> GSHMRFDEFGNIITDSAVAEEPEPELPGVTEEALRLKEAALEELAAQEVTAPLVPLAVSAFLTSRKKAAAAELADWMQSPEGQASSLESIGRSLSRRNHGRSRAVVLAHDHDEAIKGLRAVAAGKQAPNVFSVDGPVTTGPVWVLAGFGAQHRKMGKSLYLRNEVFAAWIEKVDALVQDELGYSVLELILDDAQDYGIETTQVTIFAIQIALGELLRHHGAKPAAVIGQSLGEAASAYFAGGLSLRDATRAICSRSHLMGEGEAMLFGEYIRLMALVEYSADEIREVFSDFPDLEVCVYAAPTQTVIGGPPEQVDAILARAEAEGKFARKFATKGASHTSQMDPLLGELTAELQGIKPTSPTCGIFSTVHEGRYIKPGGEPIHDVEYWKKGLRHSVYFTHGIRNA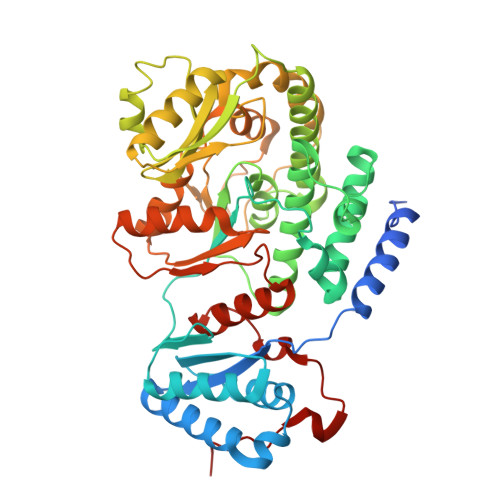VDSGHTTFLELAPNPVALMQVALTTADAGLHDAQLIPTLARKQDEVSSMVSTMAQLYVYGHDLDIRTLFSRASGPQDYANIPPTRF> MGFKLVGFSKFVRKNPKSDKFKVKRFHHIEFWCGDATNVARRFSWGLGMRFSAKSDLSTGNMVHASYLLTSGDLRFLFTAPYSPSLSAGEIKPTTTASIPSFDHGSCRSFFSSHGLGVRAVAIEVEDAESAFSISVANGAIPSSPPIVLNEAVTIAEVKLYGDVVLRYVSYKAEDTEKSEFLPGFERVEDASS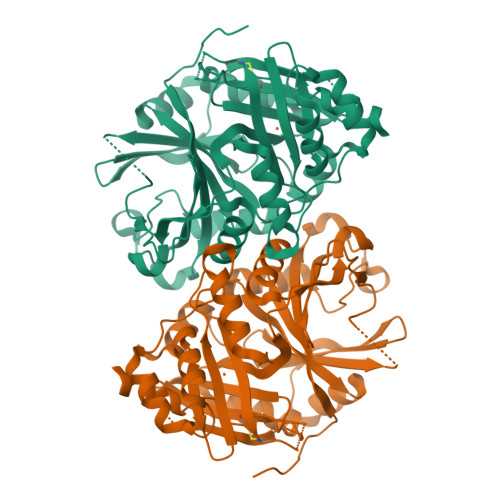FPLDYGIRRLDHAVGNVPELGPALTYVAGFTGFHQFAEFTADDVGTAESGLNSAVLASNDEMVLLPINEPVHGTKRKSQIQTYLEHNEGAGLQHLALMSEDIFRTLREMRKRSSIGGFDFMPSPPPTYYQNLKKRVGDVLSDDQIKECEELGILVDRDDQGTLLQIFTKPLGDRPTIFIEIIQRVGCMMKDEEGKAYQSGGCGGFGKGNFSELFKSIEEYEKTLEAKQLVG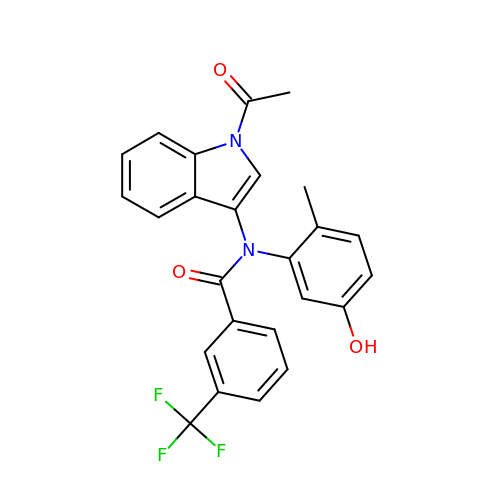N-(1-acetyl-1H-indol-3-yl)-N-(5-hydroxy-2-methylphenyl)-3-(trifluoromethyl)benzamide | C25 H19 F3 N2 O3 | GRQZQCNAGDASPY-UHFFFAOYSA-N>MLESKLKAPVFTATTQGDHYGEFVLEPLERGFGVTLGNPLRRILLSSIPGTAVTSVYIEDVLHEFSTIPGVKEDVVEIILNLKELVVRFLDPKMASTTLILRAEGPKEVRAGDFTPSADVEIMNPDLHIATLEEGGKLYMEVRVDRGVGYVPAERHGIKDRINAIPVDAIFSPVRRVAFQVEDTRLGQRTDLDKLTLRIWTDGSVTPLEALNQAVAILKEHLNYFANPEASLLPTPEVSKGEKRESAEEDLDLPLEELGLSTRVLHSLKEEGIESVRALLALNLKDLRNIPGIGERSLEEIRQALAKKGFTLKE[4x];>MEIKRFGRIREVIPLPPLTEIQVESYKKALQADVPPEKRENVGIQAAFKETFPIEEGDKGKGGLVLDFLEYRIGDPPFSQDECREKDLTYQAPLYARLQLIHKDTGLIKEDEVFLGHLPLMTEDGSFIINGADRVIVSQIHRSPGVYFTPDPARPGRYIASIIPLPKRGPWIDLEVEASGVVTMKVNKRKFPLVLLLRVLGYDQETLVRELSAYGDLVQGLLDEAVLAMRPEEAMVRLFTLLRPGDPPKKDKALAYLFGLLADPKRYDLGEAGRYKAEEKLGVGLSGRTLVRFEDGEFKDEVFLPTLRYLFALTAGVPGHEVDDIDHLGNRRIRTVGELMADQFRVGLARLARGVRERMVMGSPDTLTPAKLVNSRPLEAALREFFSRSQLSQFKDETNPLSSLRHKRRISALGPGGLTRERAGFDVRDVHRTHYGRICPVETPEGANIGLITSLAAYARVDALGFIRTPYRRVKNGVVTEEVVYMTASEEDRYTIAQANTPLEGDRIATDRVVARRRGEPVIVAPEEVEFMDVSPKQVFSLNTNLIPFLEHDDANRALMGSNMQTQAVPLIRAQAPVVMTGLEERVVRDSLAALYAEEDGEVVKVDGTRIAVRYEDGRLVEHPLRRYARSNQGTAFDQRPRVRVGQRVKKGDLLADGPASEEGFLALGQNVLVAIMPFDGYNFEDAIVISEELLKRDFYTSIHIERYEIEARDTKLGPERITRDIPHLSEAALRDLDEEGIVRIGAEVKPGDILVGRTSFKGEQEPSPEERLLRSIFGEKARDVKDTSLRVPPGEGGIVVGRLRLRRGDPGVELKPGVREVVRVFVAQKRKLQVGDKLANRHGNKGVVAKILPVEDMPHLPDGTPVDVILNPLGVPSRMNLGQILETHLGLAGYFLGQRYISPVFDGATEPEIKELLAEAFNLYFGKRQGEGFGVDKREKEVLARAEKLGLVSPGKSPEEQLKELFDLGKVVLYDGRTGEPFEGPIVVGQMFIMKLYHMVEDKMHARSTGPYSLITQQPLGGKAQFGGQRFGEMEVWALEAYGAAHTLQEMLTIKSDDIEGRNAAYQAIIKGEDVPEPSVPESFRVLVKELQALALDVQTLDEKDNPVDIFEGLASKR[2x];>MKKEVRKVRIALASPEKIRSWSYGEVEKPETINYRTLKPERDGLFDERIFGPIKDYECACGKYKRQRFEGKVCERCGVEVTRSIVRRYRMGHIELATPAAHIWFVKDVPSKIGTLLDLSATELEQVLYFNKYIVLDPKGAVLDGVPVEKRQLLTDEEYRELRYGKQETYPLPAGVDALVKDGEEVVKGQELAPGVVSRMDGVALYRFPRRVRVDYLRKERAALRIPLSAWVEKEAYRPGEVLAELSEPYLFRAEESGVVELKDLAEGHLIYLRQEEEVVARYFLPAGMTPLVVEGEIVEVGQPLAEGKGLLRLPRHMTAKEVEAEEEGDSVHLTLFLEWTEPKDYKVAPHMNVIVPEGAKVQAGEKIVAAIDPEEEVIAEAEGVVHLHEPASILVVKARVYPFEDDVEVTTGDRVAPGDVLADGGKVKSEIYGRVEVDLVRNVVRVVESYDIDARMGAEAIQELLKELDLEKLERELLEEMKHPSRARRAKARKRLEVVRAFLDSGNRPEWMILEAVPVLPPDLRPMVQVDGGRFATSDLNDLYRRLINRNNRLKKLLAQGAPEIIIRNEKRMLQEAVDAVIDNGRRGSPVTNPGSERPLRSLTDILSGKQGRFRQNLLGKRVDYSGRSVIVVGPQLKLHQCGLPKRMALELFKPFLLKKMEEKAFAPNVKAARRMLERQRDIKDEVWDALEEVIHGKVVLLNRAPTLHRLGIQAFQPVLVEGQSIQLHPLVCEAFNADFDGDQMAVHVPLSSFAQAEARIQMLSAHNLLSPASGEPLAKPSRDIILGLYYITQVRKEKKGAGMAFATPEEALAAYERGEVALNAPIVVAGRETSVGRLKFVFANPDEALLAVAHGLLDLQDVVTVRYLGRRLETSPGRILFARIVGEAVGDEKVAQELIQMDVPQEKNSLKDLVYQAFLRLGMEKTARLLDALKYYGFTLSTTSGITIGIDDAVIPEEKQRYLEEADRKLRQIEQAYEMGFLTDRERYDQVIQLWTETTEKVTQAVFKNFEENYPFNPLYVMAQSGARGNPQQIRQLCGMRGLMQKPSGETFEVPVRSSFREGLTVLEYFISSHGARKGGADTALRTADSGYLTRKLVDVAHEIVVREADCGTTNYISVPLFQMDEVTRTLRLRKRSDIESGLYGRVLAREVEALGRRLEEGRYLSLEDVHFLIKAAEAGEVREVPVRSPLTCQTRYGVCQKCYGYDLSMARPVSIGEAVGVVAAESIGEPGTQLTMRTFHTGGVAVGTDITQGLPRVIELFEARRPKAKAVISEIDGVVRIEEGEDRLSVFVESEGFSKEYKLPKDARLLVKDGDYVEAGQPLTRGAIDPHQLLEAKGPEAVERYLVDEIQKVYRAQGVKLHDKHIEIVVRQMLKYVEVTDPGDSRLLEGQVLEKWDVEALNERLIAEGKVPVAWKPLLMGVTKSALSTKSWLSAASFQNTTHVLTEAAIAGKKDELIGLKENVILGRLIPAGTGSDFVRFTQVVDQRTLKAIEEARKEAVEAKEKEAPRRPVRREQPGKGL[2x];>MAEPGIDKLFGMVDSKYRLTVVVAKRAQQLLRHRFKNTVLEPEERPKMRTLEGLYDDPNAVTWAMKELLTGRLFFGENLVPEDRLQKEMERLYPTEEEA[2x];>TSDPVRQYLHEIGQVPLLTLEEEIDLARKVEEGMEAIKKLSEATGLDQELIREVVRAKILGTARIQKIPGLKEKPDPKTVEEVDGKLKSLPKELKRYLHIAREGEAARQHLIEANLRLVVSIAKKYTGRGLSFLDLIQEGNQGLIRAVEKFEYKRRFKFSTYATWWIRQAINRAIADQARTIRIPVHMVETINKLSRTARQLQQELGREPSYEEIAEAMGPGWDAKRVEETLKIAQEPVSLETPIGDEKDSFYGDFIPDENLPSPVEAAAQSLLSEELEKALSKLSEREAMVLKLRKGLIDGREHTLEEVGAYFGVTRERIRQIENKALRKLKYHESRTRKLRDFLE[2x];>[2x]MKEFRPGDKVVLPPYGVGVVAGIAQRSVSGVSRAYYQVDFPGSRSKAYVPVEAPHSVGLRKALAPEEVPVILDLLKNGRMPLPKQWAARHRKTSEILADGNPYRIAQMAGQLRAWEVERGLPDLDRQALRRAIHLLAEEVAQSLEITVQEAKRLFEEAWGEELN

CarD, first identified as a regulator of ribosomal RNA (rRNA) transcription in Mycobacterium tuberculosis (Mtb), is a transcriptional activator widely distributed among bacterial species, including Thermus species, but is absent in Eco. CarD is a global regulator that is an essential protein in Mtb, the causative agent of tuberculosis. Crystal structures of Tth and Mtb CarD reveal an N-terminal domain with a Tudor-like fold (CarD-RID, RNAP interacting domain) in common with the Eco transcription repair coupling factor (TRCF)-RID, and a helical C-terminal domain (CarD-CTD). The structural results, combined with supporting biochemical studies, establish that the CarD-RID makes a protein/protein interaction with the RNAP β1-lobe, thereby positioning the CarD-CTD and a conserved Trp residue to interact with the upstream edge of the transcription bubble, using a wedge mechanism to prevent collapse of the transcription bubble.

Crystals of CarD transcription activation complexes were prepared by soaking Tth CarD into Taq Δ1.1σA-holoenzyme/us-fork (−12 bp) or full RPo crystals. The structures of CarD transcription activation complexes were refined to 4.4 and 4.3 Å-resolution, respectively. The protein/protein and protein/nucleic acid interactions were essentially identical among all of the four crystallographically independent complexes, so the more complete and higher resolution CarD/RPo structure is described here. CarD does not make significant interactions with σA but interacts with the promoter DNA from −14 to −10 from the opposite, (distorted) minor groove side of the DNA such that the σA/DNA interactions and the structure of the transcription bubble in RPo and CarD/RPo are essentially the same. The N-terminal ends of two CarD-CTD α-helices (α3 and α5) make direct contacts with the promoter DNA. The peptide backbone nitrogen of CarD-L124, at the N-terminal end of α5, closely approaches the backbone phosphate oxygen of the template strand (t-strand) at the −14 position [−14(t)], possibly forming a hydrogen bond, an interaction likely facilitated by the partial positive charge of the α5 helix dipole. The bulky, hydrophobic planar side chain of W86, located at the N-terminal end of α3, wedges into the splayed minor groove at the upstream edge of the transcription bubble. Despite the relatively low resolution of our analysis, CarD-W86 was clearly resolved in electron density maps. The mode of CarD/DNA interaction is incompatible with duplex B-form DNA; the normal minor groove is too narrow to accommodate the end of CarD-α3 and CarD-W86. The minor groove W-wedge increases the lifetime of RPo by preventing transcription bubble collapse.4-benzylpiperazine-2,6-dione | C11 H12 N2 O2 | 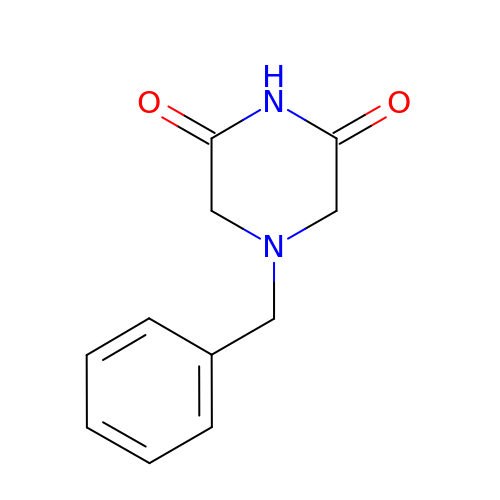VURIYIYAKMLWMZ-UHFFFAOYSA-N> PISPIETVPVKLKPGMDGPKVKQWPLTEEKIKALVEICTEMEKEGKISKIGPENPYNTPVFAIKKKDSTKWRKLVDFRELNKRTQDFWEVQLGIPHPAGLKKKKSVTVLDVGDAYFSVPLDEDFRKYTAFTIPSINNETPGIRYQYNVLPQGWKGSPAISQSSMTKILEPFKKQNPDIVIYQYMDDLYVGSDLEIGQHRTKIEELRQHLLRWGLTTPDKKHQKEPPFLWMGYELHPDKWTVQPIVLPEKDSWTVNDIQKLVGKLNWASQIYPGIKVRQLSKLLRGTKALTEVIPLTEEAELELAENREILKEPVHGVYYDPSKDLIAEIQKQGQGQWTYQIYQEPFKNLKTGKYARMRGAHTNDVKQLTEAVQKITTESIVIWGKTPKFKLPIQKETWETWWTEYWQATWIPEWEFVNTPPLVKLWYQLEKEPIVGAETFYVDGAANRETKLGKAGYVTNKGRQKVVPLTNTTNQKTELQAIYLAL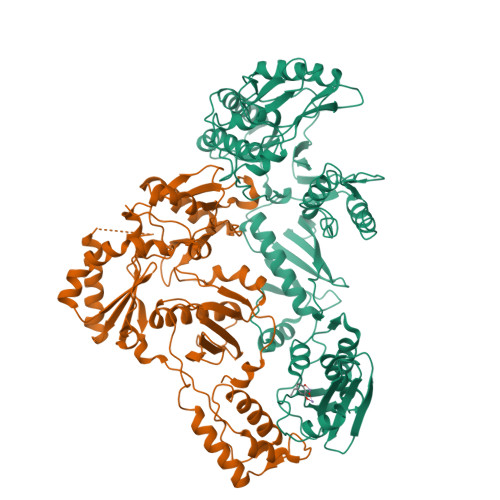QDSGLEVNIVTDSQYALGIIQAQPDKSESELVNQIIEQLIKKEKVYLAWVPAHKGIGGNEQVDKLVSAG;> PISPIETVPVKLKPGMDGPKVKQWPLTEEKIKALVEICTEMEKEGKISKIGPENPYNTPVFAIKKKDSTKWRKLVDFRELNKRTQDFWEVQLGIPHPAGLKKKKSVTVLDVGDAYFSVPLDEDFRKYTAFTIPSINNETPGIRYQYNVLPQGWKGSPAIFQSSMTKILEPFKKQNPDIVIYQYMDDLYVGSDLEIGQHRTKIEELRQHLLRWGLTTPDKKHQKEPPFLWMGYELHPDKWTVQPIVLPEKDSWTVNDIQKLVGKLNWASQIYPGIKVRQLSKLLRGTKALTEVIPLTEEAELELAENREILKEPVHGVYYDPSKDLIAEIQKQGQGQWTYQIYQEPFKNLKTGKYARMRGAHTNDVKQLTEAVQKITTESIVIWGKTPKFKLPIQKETWETWWTEYWQATWIPEWEFVNTPPLVKLWYQ> FNKIKDSVKQKIDSMGDKGTYGVSASHPLAVEEGMKVLKNGGSAVDAAIVVSYVLGVVELHASGIGGGGGMLIISKDKETFIDYRETTPYFTGNQKPHIGVPGFVAGMEYIHDNYGSLPMGELLQPAINYAEKGFKVDDSLTMRLDLAKPRIYSDKLSIFYPNGEPIETGETLIQTDLARTLKKIQKEGAKGFYEGGVARAISKTAKISLEDIKGYK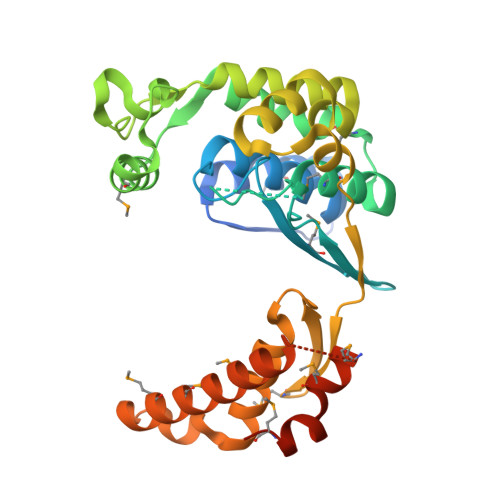VEVRKPVKGNYMGYDVYTAPPPFSGVTLLQMLKLAEKKEVYKDVDHTATYMSKMEEISRIAYQDRKKNLGDPNYVNMDPNKMVSDKYISTMKNENGDALSEAEHES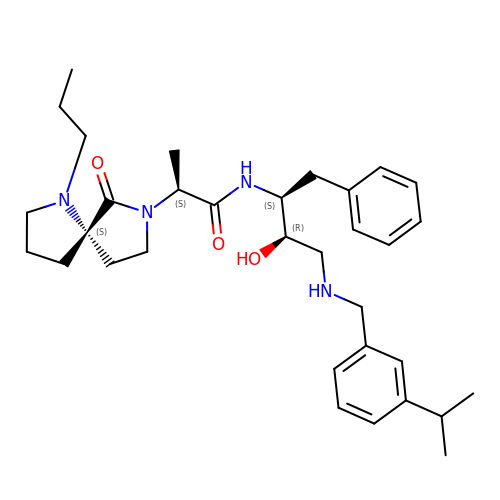(2S)-N-[(2S,3R)-3-hydroxy-1-phenyl-4-{[3-(propan-2-yl)benzyl]amino}butan-2-yl]-2-[(5S)-6-oxo-1-propyl-1,7-diazaspiro[4.4]non-7-yl]propanamide | C33 H48 N4 O3 | MOXAMLWWFJKUEH-XGZLTPBASA-N> MTARIALASLFVVAAVLAQPWQTTTQRWVLGVSIAAVIVLLAWWKGMFLTTRIGRALAMVRRNRAEDTVETDAHRATVVLRVDPAAPAQLPVVVGYLDRYGITCDKVRITHRDAGGTRRSWISLTVDAVDNLAALQARSARIPLQDTTEVVGRRLADHLREQGWTVTVVEGVDTPLPVSGKETWRGVADDAGVVAAYRVKVDDRLDEVLAEIGHLPAEETWTALEFTGSPAEPLLTVCAAVRTSDRPAAKAPLAGLTPARGRHRPALAALNPL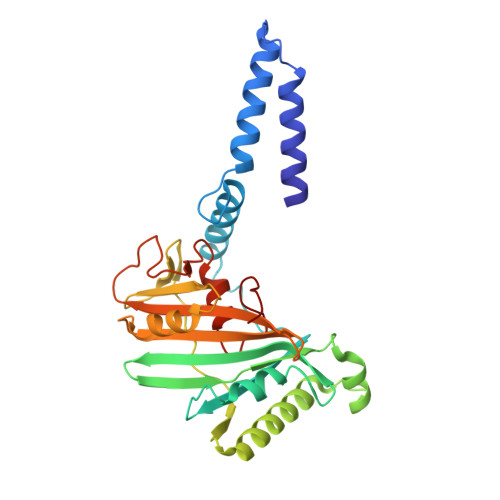STERLDGTAVPL N-hydroxy-2-[(6-oxo-4-phenyl-1,6-dihydropyrimidin-2-yl)sulfanyl]acetamide | C12 H11 N3 O3 S | 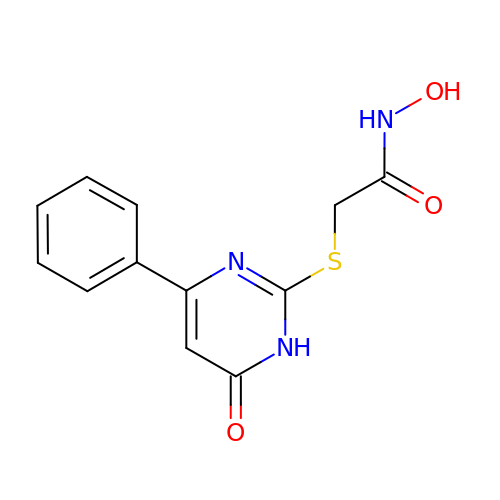HEUAAARBOBGFCJ-UHFFFAOYSA-N>[11x]NFTAPVTTPSIPTPIQFLQTWLPGFVKVMTAARKIDEIIGIDTVGSWEDQEIVQGIVEPAGTAVEYGDHTNIPLTSWNANFERRTIVRGELGMMVGTLEEGRASAIRLNSAETKRQQAAIGLETFRNAIGFYGWQSGLGNRTYGFLNDPNLPAFQTPPSQGWSTADWAGIIGDIREAVRQLRIQSQDQIDPKAEKITLALATSKVDYLSVTTPYGISVSDWIEQTYPKMRIV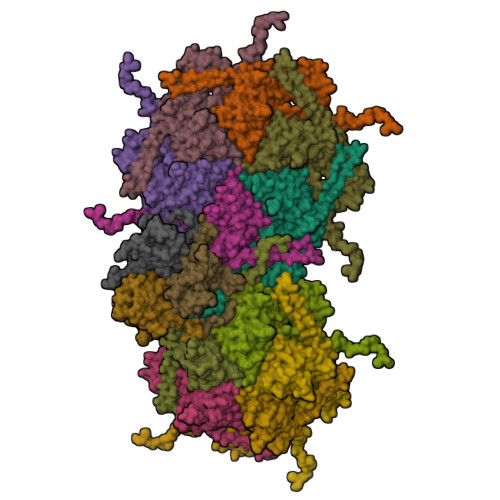SAPELSGVQMKNQEPEDALVLFVEDVNAAVDGSTDGGSVFSQLVQSKFITLGVEKRAKSYVEDFSNGTAGALCKRPWAVVRYLGI;>MFQKQVYRQYTPGFPGDLIEDGPKRARPGRIMSLSAVNPAATATGPNRASRAFGYAGDVSALGEGQPKTIAARASEVVIGGANFFGVLGHPKHYALFGSAGDSLAPSYDLPDGAEGEFFDMATGLVVEIFNGAAAALDLDYGDLVAYVPNNLATADDALGLPAGALVGFKTGSMPTGLVQIPNARIVNAISLPAQSAGNLVAGVTIVQLTQ[3x]pretilachlor | C17 H26 Cl N 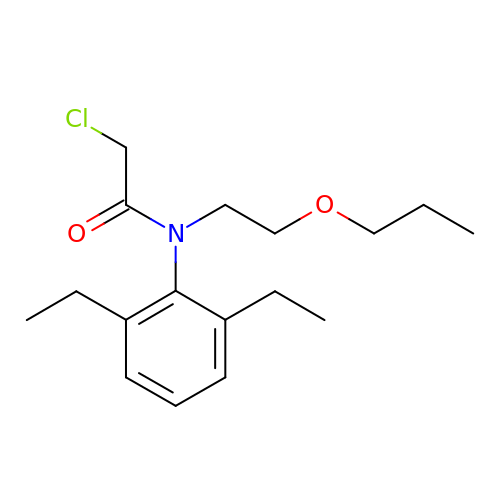O2 | YLPGTOIOYRQOHV-UHFFFAOYSA-N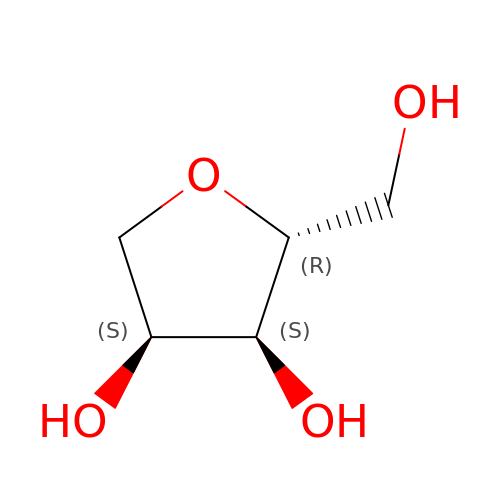1,4-anhydro-D-ribitol | C5 H10 O4 | KZVAAIRBJJYZOW-LMVFSUKVSA-N> SNEFTYSYLFRMISHEMKQKADQKLEQFDITNEQGHTLGYLYAHQQDGLTQNDIAKALQRTGPTVSNLLRNLERKKLIYRYVDA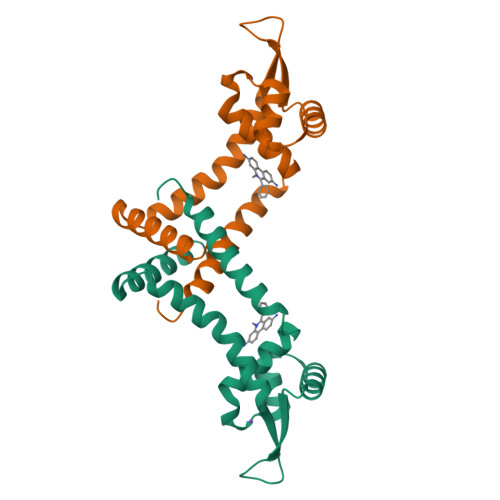QDTRRKNIGLTTSGIKLVEAFTSIFDEMEQTLVSQLSEEENEQMKANLTKMLSSLQ> GSHMRLGAQSIQPTANLDRTDDLVYLNVMELVRAVLELKNELAQLPPEGYVVVVKN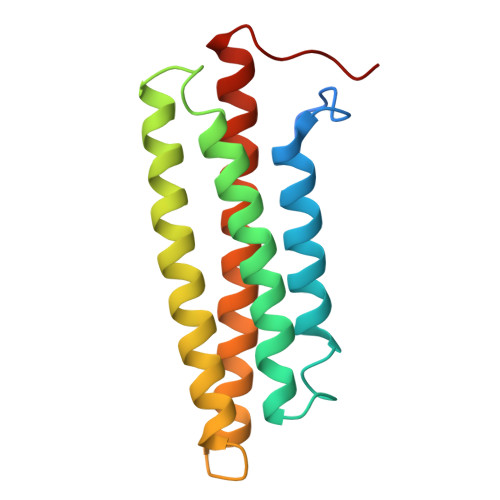VGLTLRKLIGSVDDLLPSLPSSSRTEIEGTQKLLNKDLAELINKMRLAQQNAVTSLSEECKRQMLTASHTLAVDAKNLLDAVDQAKVLANLAHPPAE>[2x]MAYVPLSGTNVRILADVPFSNDYKNTRWFTSSSNQYNWF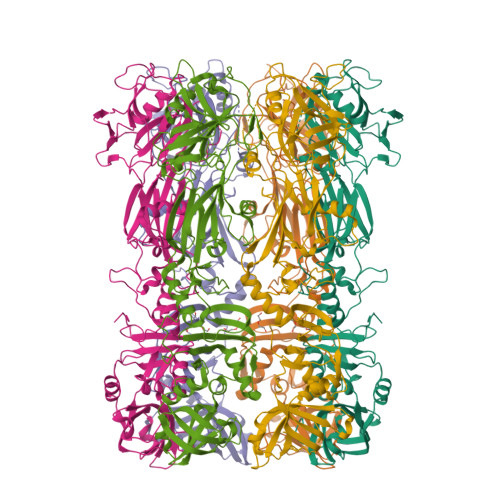NSKSRVYEMSKVTFMGFRENKPYVSVSLPIDKLYSASYIMFQNADYGNKWFYAFVTELEFKNSAVTYVHFEIDVLQTWMFDIKFQESFIVREHVKLWNDDGTPTINTIDEGLSYGSEYDIVSVENHKPYDDMMFLVIISKSIMHGTPGEEESRLNDINASLNGMPQPLCYYIHPFYKDGKVPKTYIGDNNANLSPIVNMLTNIFSQKSAVNDIVNMYVTDYIGLKLDYKNGDKELKLDKDMFEQAGIADDKHGNVDTIFVKKIPDYEALEIDTGDKWGGFTKDQESKLMMYPYCVTEITDFKGNHMNLKTEYINNSKLKIQVRGSLGVSNKVAYSVQDYNADSALSGGNRLTASLDSSLINNNPNDIAILNDYLSAYLQGNKNSLENQKSSILFNGIMGMIGGGISAGASAAGGSALGMASSVTGMTSTAGNAVLQMQAMQAKQADIANIPPQLTKMGGNTAFDYGNGYRGVYVIKKQLKAEYRRSLSSFFHKYGYKINRVKKPNLRTRKAFNYVQTKDCFISGDINNNDLQEIRTIFDNGITLWHTDNIGNYSVENELRHHHHHH(2,5-dihydro-1H-pyrrol-1-yl)(2',6-dimethyl[1,1'-biphenyl]-3-yl)methanone | C19 H19 N O | 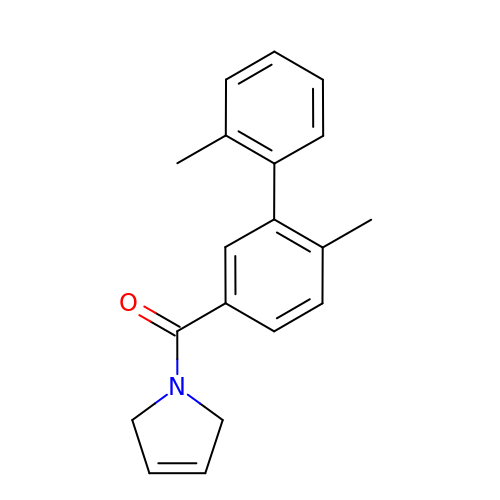NIOIWNZLGVRPNS-UHFFFAOYSA-N Interleukin 4 (IL-4) is a pleiotropic cytokine that plays a major regulatory role in the immune system. Signal transduction of IL-4 is mediated by a sequential binding process, initiated first by binding of IL-4 to its high-affinity single membrane spanning receptor chain IL-4Rα. This intermediate ligand receptor complex then recruits one of two possible low-affinity receptor subunits, the common gamma chain (γc) or the IL-13Rα1 chain, into the functional hetero-trimeric complex to initiate signalling. The overall structure of IL-4 comprises the known four-helical bundle in up-up-down-down topology, which like the crystal packing is unaffected by these mutations.

The structures of the IL-4 variants T13D (max. resolution 1.65 Å), F82D (max. resolution 1.7Å) and T13D-F82D (max. resolution 1.8Å) were refined on the basis of the structure of wild-type IL-4 (max. resolution 1.8Å); all crystals were obtained under identical conditions, allowing detailed comparison. For comparison, in the structure of wild-type IL-4, the hydroxyl group of Thr13 is hydrogen-bonded to the main chain carbonyl of Glu9; the side chain of Arg85 is moved outward towards the solvent and fixed to the hydroxyl group of Thr13 by a water-mediated H-bond. The change in side chain conformation of Arg85 becomes clear if the side chain torsion angles of the wild-type and variant are compared. The χ1 torsion angle of Arg85 is in the trans conformation (174° IL-4, 176° IL-4 T13D) for both proteins; in the case of IL-4, χ2 of Arg85 is slightly off trans (160°), whereas for T13D, the torsion angle χ2 of Arg85 is in the trans conformation (176°). In contrast, the χ3 torsion angle differs by 115° between IL-4 (58°, gauche- conformation) and T13D (-57°, gauche+ conformation). In contrast, in our current study, the temperature factors for the side chain atoms of Arg85 are of similar magnitude in the high-resolution structures of wild-type IL-4 (mean 23Å2 for side chain from Cβ) and its variant T13D (mean 20Å2). These values are also close to those of the atoms located in the hydrophobic core (mean 15Å2), therefore the side chain of Arg85 can be considered rigid. Cluster III consists of the positively charged residues Arg81 and Arg85 of IL-4 and the negatively charged residues Asp66, Asp67 and Asp125 of IL-4Rα. Arg81 and Arg85 of IL-4 form several hydrogen bonds with residues of IL-4Rα; however, these interactions do not seem productive. Therefore, the conformational entropy is not decreased for Arg85 in the formation of the T13D-IL-4Rα complex, whereas for wild-type IL-4 the side chain of Arg85 becomes ordered only upon binding to IL-4Rα.

> HKCDITLQEIIKTLNSLTEQKTLCTELTVTDIFAASKNTTEKETFCRAATVLRQFYSHHEKDTRCLGATAQQFHRHKQLIRFLKRLDRNLWGLAGLNSCPVKEANQSTLENFLERLKTIMREKYSKCSS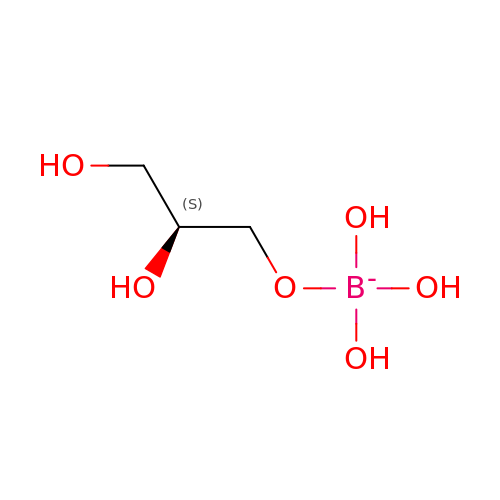(S)-(2,3-DIHYDROXYPROPOXY)TRIHYDROXYBORATE | C3 H10 B O6 | KLKDDPLTQSQDLA-VKHMYHEASA-N>MRGSHHHHHHGSNVAKNNLKNNKDIERKEKIIILGSGWGGFNFLLNIDFKKYDVTLISPRNYFTFTPLLPCLCSGTLSVNVCTESIRNFLRKKNGYCGNYLQLECTDVFYEDKYINCIDIENNKVKLFYDYLIIAVGAKTNTFNINGVDKYAYFVKDIDDALKIRKKFLDILEKCTLPNISNEEKKKMLHVAVVGGGPTGVEVTAEFADFINKEVKINYKDIFNFISISIIEGGNNLLPTFTQNISDFTKENFHNLNINVLTNYYVIDVDKHSFHIQSSLNKNEKKKLSYGLLIWASGLAQTTLIQKFLKTIPVQANNAILKVDEKLRVIGIPSNNIYAIGDCKKIQPKLLHEHTNEIIKILTGNKLTSEALKLKQSELTKTFPQLSISKWDYEKNKKGEMTPQQFHD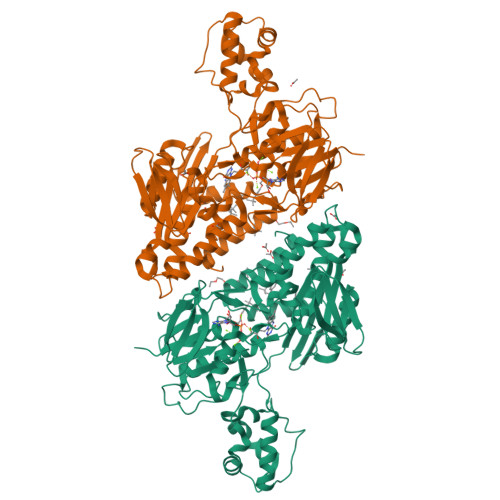YLFEIDKNYKSPTPTAQNAKQEAYYLSNVFNNFIHTNQKFNIPSFIEKWKGSLAYIGNHQVVADLPYYELKGGRFSSTFWKVVYIQLLLSWKSRFHFFIDFIKTKWYGRPFIK[2x]10-oxooctadecanoic acid | C18 H34 O3 | 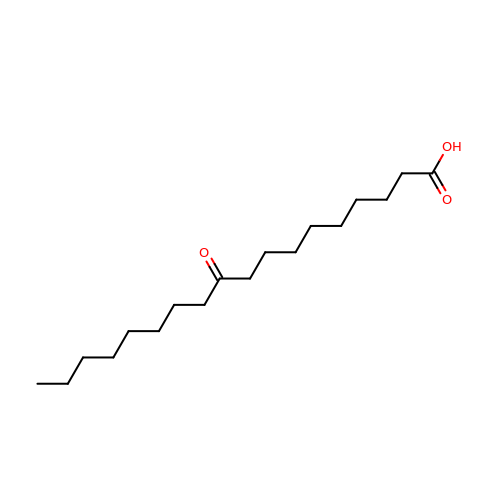BGKROBBCCGUUCF-UHFFFAOYSA-N P. stutzeri WM88 has PtxABC, HtxBCDE and PhnCDE ABC-transporters for the acquisition of phosphite, hypophosphite and organophosphonates, respectively. These transport systems rely on a high-affinity periplasmic binding protein (PBP) to impart ligand specificity. HtxB is a typical type-II PBP, with a binding pocket positioned in a deep groove between two domains separated by a hinge region. A comparison of the HtxB and PtxB structures showed that sequence differences within the binding pocket essentially eliminate an oxygen binding site in HtxB, providing specificity for a ligand with two oxygen atoms (hypophosphite), over one with three (phosphite).

In the HtxB complex with phosphite, the phosphorus centre of the ligand and the four tetrahedral atoms surrounding it (3 oxygen and 1 hydrogen) occupy approximately the same positions as the equivalent atoms in the hypophosphite complex (2 oxygen and 2 hydrogen). The two common oxygen atom positions between the phosphite and hypophosphite make equivalent interactions with residues in the binding pocket, namely the sidechain and mainchain amide of T129, S130, the sidechain hydroxyl of Y97 and the structural water molecule (HOH). The pocket is capped by a tryptophan sidechain (W52) that makes a P-H…π interaction with the R1 hydrogen atom of the phosphite (distance of 2.7 Å and angle of approximately 140°), forming a similar interaction to that present in the hypophosphite complex. However, the additional oxygen atom of the phosphite, to which it is equivalent, points towards the D206/R178 salt bridge to one side of the HtxB binding pocket. This phosphite-oxygen atom is 2.8 Å away from the oxygen atom of D206 and 3.2 Å away from the nitrogen atom of R178, suggesting that both residues interact with this phosphite-oxygen, albeit with a rather long hydrogen bond to the arginine. Although we could not directly observed the position of the hydrogen atoms in the structure, at pH 5 it is likely that the majority of the phosphite in solution is mono-anionic (pKa 1.3, 6.7), carrying a single proton on one of the three oxygen atoms. The 2.8 Å distance between the phosphite-oxygen and D206 implies, therefore, that the phosphite is protonated at this position and acts as a hydrogen bond donor to D206. These additional hydrogen bonds appear to provide enough stabilising energy to trap a fully closed complex in the crystal structure, which is virtually identical to the conformation observed in the complex with hypophosphite (RMSD Cα: 0.25 Å). We have shown that HtxB is capable of binding phosphite at pH 5 due to a change in the protonation state of the ligand that facilitates the formation of extra hydrogen bonds within the binding pocket of the protein, enabling the formation of a closed complex. Although this complex can be captured by crystallisation with a large excess of phosphite (5 mM), the Kd of HtxB for phosphite at pH 5 is only 1.74 mM, which is ca. 1000 × less than hypophosphite at the same pH.

> MAEVVNGKLHLRFAIAPMRPTPSQTIKEFEPIFKYLADQLGATYEIVSPESWAAISVAMTNGHVDVGWLGPWGYVLSNKKAGTEVLATVKYRGEPFYKALIVGRADLPIKKWPEDAKGLKLSLSDQGNTSGWLIPMAYFKSIGIDPASYFEYREGATFGQNESQIQHGLIDLGSDMDRGRNGMIEAGQIDPSKSKIVWESSKLPNDAISVPKDFDPALKARITEILTSLSEEKAQSLMGSGYNGFVKAKHSDYKVIEDAGRILGKLLEHHHHHH> MKVLFRSDSSSQIGFGHIKRDLVLAKQYSDVSFACLPLEGSLIDEIPYPVYELSSESIYELINLIKEEKFELLIIDHYGISVDDEKLIKLETGVKILSFDDEIKPHHCDILLNVNAYAKASDYEGLVPFKCEVRCGFSYALIREEFYQEAKENRKKKYDFFICMGG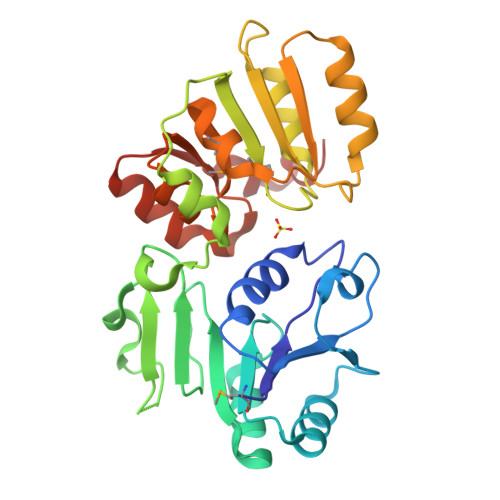TDIKNLSLQIASELPKTKIISIATSSSNPNLKKLQKFAKLHNNIRLFIDHENIAKLMNESNKLIISASSLVNEALLLKANFKAICYVKNQESTATWLAKKGYEVEYKYLEHHHHHH> ANATVKMGSDSGALVFEPSTVTIKAGEEVKWVNNKLSPHNIVFDADGVPADTAAKLSHKGLLFAAGESFTSTFTEPGTYTYYCEPHRGAG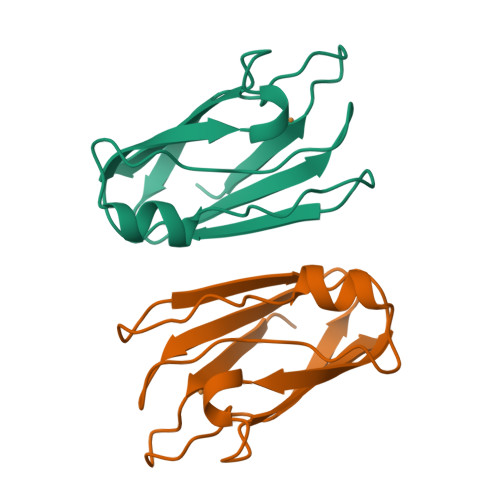MVGKVVVE>TTGHSYEKYNNWETIEAWTKQVTSENPDLISRTAIGTTFLGNNIYLLKVGKPGPNKPAIFMDCGFHAREWISHAFCQWFVREAVLTYGYESHMTEFLNKLDFYVLPVLNIDGYIYTWTKNRMWRKTRSTNAGTTCIGTDPNRNFDAGWCTTGASTDPCDETYCGSAAESEKETKALADFIRNNLSSIKAYLTIHSYSQMILYPYSYDYKLPENNAELNNLAKAAVKELATLYGTKYTYGPGATTIYPAAGGSDDWAYDQGIKYSFTFELRDKGRYGFILPESQIQATCEE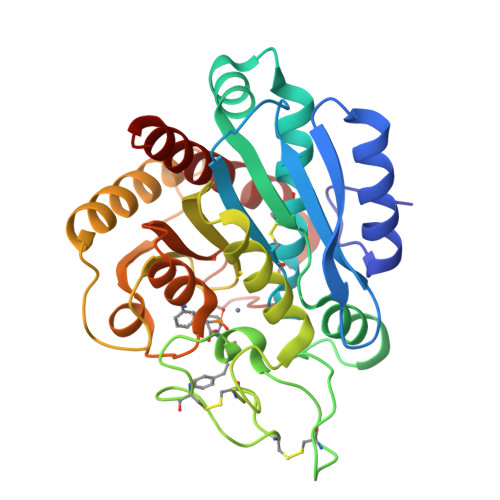TMLAIKYVTNYVLGHL[3x]There is a family of proteins that have been shown to enable growth of differentially culturable mycobacteria. These proteins, known as resuscitation-promoting factors (Rpfs), are a class of cell wall remodelling enzymes called lytic transglycosylases (Ltgs) which are ubiquitous to bacteria and some bacteriophages. Ltgs cleave the β-1,4 glycosidic bond between alternating N-Acetylmuramic acid (MurNAc) and N-Acetyl-D-glucosamine (GlcNAc) residues that make up the peptidoglycan backbone. We focused our studies on one of these proteins, LtgG (BPSL3046). The presence of multiple Ltgs may suggest functional redundancy, however the results of this study demonstrate that LtgG has specific roles in cell division, motility and virulence of B. pseudomallei.

Crystals of LtgG were grown at pH 7.5 and diffracted to 1.73 Å resolution. LtgG is comprised of two domains, a large β-barrel domain and a smaller α-/β-domain that is an insert of the larger domain. Residues proposed to form part of the catalytic site in the E. coli protein, including the catalytic aspartate (Asp343 in LtgG), together with threonine (Thr128) and tyrosine (Tyr130) residues are conserved in LtgG, suggesting a common catalytic mechanism. Most notably, the binding groove is narrower in the substrate bound structure, allowing interactions with both domains. To confirm that the aspartate at position 343 was catalytically important, we generated a Asp343Ala (D343A) mutant protein. The mutant eluted from the gel-filtration column at the same position as the wild-type enzyme indicating that it was folded correctly. Zymograms performed using equivalent concentrations of the wildtype and mutant proteins reveal a complete loss of muralytic activity as a result of the mutation, indicated by an absence of clearance under established conditions appropriate for wildtype LtgG. The D343A mutation completely abolished the complementation of cellular morphology in ∆ltgGCFD. Thus, our results proved that muralytic activity of LtgG was required for its function in B. pseudomallei.

> GSPVRQGARPAGAAIVPGQIAAARLTPVAWQQVPGWQDDSLIGATIALRQNCARLARQANWQRACAAAMRLDDLDVGSARTFFETYFTPFQFANNDGTLDGLVTGYYEPLLHGSRVRRGPYQYALYRWPAGYRAGASMPARAQLMRSGALSGNELVWVDDPIEAFFLQVQGSGRVVLDDGTVMRVGYGGTNNQPYRSIGKWLLDHGELGAGQATMQGIKAWARANPSRVDALLDTNPRFVFFREMPSQEDVPHGGADGPVGALGVPLTPERSIAVDPSSIPLGTPVFLQTTRPMTNAPLNRLVFAQDVGTAIKGGVRADYFWGLGDDAGDQAGRMKQNGRMWLLFPNS>NDFHRDTWAEVDLDAIYDNVENLRRLLPDDTHIMAVVKANAYGHGDVQVARTALEAGASRLAVAFLDEALALREKGIEAPILVLGASRPADAALAAQQRIALTVFRSDWLEEASALYSGPFPIHFHLKMDTGMGRLGVKDEEETKRIVALIERHPHFVLEGLYT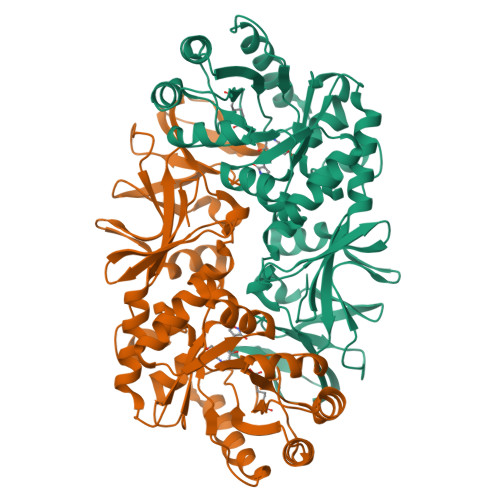HFATADEVNTDYFSYQYTRFLHMLEWLPSRPPLVHCANSAASLRFPDRTFNMVRFGIAMYGLAPSPGIKPLLPYPLKEAFSLHSRLVHVKKLQPGEKVSYGATYTAQTEEWIGTIPIGYADGWLRRLQHFHVLVDGQKAPIVGRICMDQCMIRLPGPLPVGTKVTLIGRQGDEVISIDDVARHLETINYEVPCTISYRVPRIFFRHKRIMEVRNAIGRGESSA[2x]> SMLSSRNRPEGKVLETVGVFEVPKQNGKYETGQLFLHSIFGYRGVVLFPWQARLYDRDVASAAPEKAENPAGHGSKEVKGKTHTYYQVLIDARDCPHISQRSQTEAVTFLANHDDSRALYAIPGLDYVSHEDILPYTSTDQVPIQHELFERFLLYDQTKAPPFVARETLRAWQEKNHPWLELSDVHRETTENIRVTVIPFYMGMREAQNSHVYWWRYCIRLENLDSDVVQLRERHWRIFSLSGTLETVRGRGVVGREPVLSKEQPAFQYSSHVSLQASSGHMWGTFRFERPDGSHFDVRIPPFSLESNKDEKTPPSGLHW

Polymerase δ‐interacting protein 2 (POLDIP2, PDIP38) is a multifaceted, “moonlighting” protein, involved in binding protein partners from many different cellular processes, including mitochondrial metabolism and DNA replication and repair. 4 This is followed by two predicted globular YccV and ApaG/DUF525 domains, with putative functions in bacterial homologues of hemi‐methylated DNA binding (YccV) 5 and nucleotide binding (ApaG). 7 , 8 POLDIP2 stimulates Polδ by increasing its binding to PCNA, a homotrimeric ring‐shaped processivity factor for DNA synthesis, 7 potentially by bridging the molecules, with the POLDIP2 NTD required for full stimulation. 9 POLDIP2 directly stimulates PrimPol DNA binding, synthesis and processivity during translesion bypass.

Here we report the crystal structure of the POLDIP251‐368 fragment to 2.8 Å, demonstrating that it has a rigid core structure with closely packed extended YccV and DUF525 domains, confirmed by solution scattering and molecular dynamics simulations. The POLDIP251‐368 structure was solved with molecular replacement, using bacterial HspQ (YccV) 14 and human FBxo3 (DUF525), 15 with one molecule in the asymmetric unit and R work/R free factors of 0.216/0.288 respectively, 99.67% completeness and 99.6% of residues in preferred or allowed Ramachandran regions. The POLDIP251‐368 crystal structure exhibits a globular fold, with the YccV‐like and DUF525 domains juxtaposed on top of each other. The YccV‐like α1 helix leads immediately into a presumed “linker” region between the YccV and DUF525 domains, comprising the α2/310 helix (residues 201–230). Instead, we propose this region is part of an extended YccV (E‐YccV) domain. The E‐YccV domain is connected by a short linker (Ser231‐Asp232) to the DUF525 domain (residues 233–368), which exhibits a fibronectin type III/immunoglobulin (β‐sandwich) fold, comprising two opposing four‐stranded antiparallel β‐sheets. Part of the N‐terminal loop was structured in the crystal (residues 49–66), comprising the short β0 strand formed partly from Met50 (remaining following tag cleavage). β0 hydrogen bonds with the distal β15 strand of the upper β‐sheet, thereby connecting DUF525 to the N‐terminal region. On closer examination we observed an internal cavity traversing the protein at the interface (dashed boxes), lined with predominantly hydrophilic residues contributed from both E‐YccV and DUF525 domains (inset). During structural refinement we observed that Cys266 exhibited electron density that could not be accounted for, either by alternative rotamers or by surrounding residues (green). Protein mass spectrometry also confirmed the expected molecular weight, furthermore, a mass difference reflecting the size of the density was not observed (not shown). This prompted us to speculate that this could reflect an oxidized (or other) post‐crystallization modification of Cys266, given its exposure to the cellular environment via the channel.>[10x]MAHHHHHHMARNYAYPHMNTLKNKHNIMSTKKLAHVCEHYAKKAIINLNKEPLPQKFDSSYLKYIHQRLFESTFEWAGYTRDFSFTFDDGTVAEMPMMKVPNLDIFYVQGNDIQENLKKFDQLLASKNNLQGLSREEFVDEAAKLFVFLNSIAPFRAGNEPTQRVFFEKLAEAAGHQLDFSVATEKRIMRACIDGMTLKDNMAYKEMKSLFEDISDPKKIAALKNFLRRIPRLERERLNDE

Proteins containing a FIC domain catalyze AMPylation and other post-translational modifications (PTMs). Among these, Bartonella effector proteins (Beps) comprise a particularly diverse ensemble of FIC domains that subvert various host cellular functions. The FIC fold comprises eight conserved α-helices and encompasses a characteristic active site loop between helices α4 and α5 that forms most of the catalytic center and the substrate binding pocket. Additionally, FIC domains generally contain a β-hairpin between helix α2 and helix α3 that is referred to as the “flap” and mediates docking of a target segment in extended conformation via β-strand augmentation.

BepFIC domains with a glutamate (E159) in position G2 are represented by the B15_Bep8 and B11C_Bep8 structures, which are virtually identical. Although the motif is highly degenerated to PFxxGNE, the fold of the domain and, in particular, of the active loop are canonical. Nevertheless, the binding of a triphosphate-nucleotide appears to be impossible due to the presence of the side-chain in position G2 (compare Figure 9A and Figure 9B). However, simple outward rotation of the glutamate side-chain allows the accommodation of an AMPylated side-chain in a constellation very similar to that of the Tyr-AMP target side-chain in the IbpA/Cdc42 complex. Intriguingly, the model would allow binding of water molecule to the N-terminal end of α5 ready for a nucleophilic attack onto the phosphorous, which is in line with its phosphoester bond with the tyrosine, i.e., it is ready for deAMPylation of the modified side-chain. The strict conservation of a glutamate in G2 may then point to a role in water binding and proton abstraction, i.e., the glutamate would function as general base. About one quarter of BepFIC domains display a glutamate in the G2 position which would clearly interfere with the triphosphate-nucleotide binding mode observed in AMP transferases, i.e., with the γ-phosphate forming a salt-bridge with R2. However, binding of an AMPylated target to members of this group of BepFICs appears possible, which suggests that they might act as deAMPylases with the glutamate in G2 involved in binding and deprotonation of the hydrolytic water. B11C_Bep8 FIC crystals were grown from a solution of 30% (v/v) Jeffamine M-600 and 100 mM HEPES free acid/NaOH, pH 7.0. Data for Bqu_BepC FIC with ADP, Bcl_Bep1 FIC, and B11C_Bep8 FIC were collected at 100 K on a Rayonix MX-225 detector at a wavelength of 0.9786 Å on beamline 21-ID-F at the Advanced Photon Source (APS, Argonne, IL, USA).>[2x]TRDQNGTWEMESNENFEGYMKALDIDFATRKIAVRLTQTLVIDQDGDNFKTKTTSTFRNYDVDFTVGVEFDEYTKSLDNRHVKALVTWEGDVLVCVQKGEKENRGWKKWIEGNKLYLEL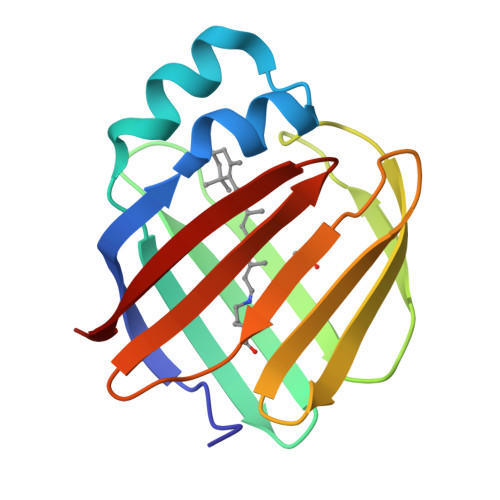TCGDQVCRQVFKKK>ASVHGTTYELLRRQGIDTVFGNPGSNELPFLKDFPEDFRYILALQEACVVGIADGYAQASRKPAFINLHSAAGTGNA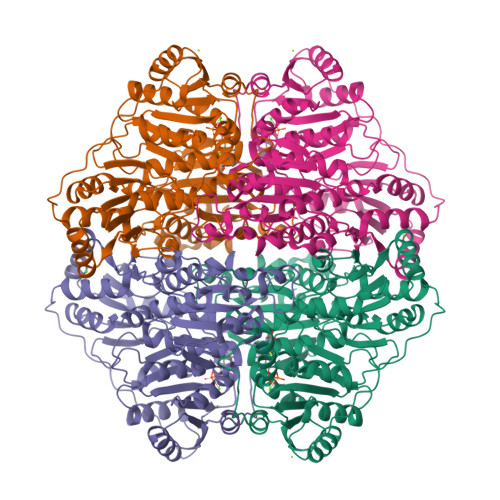MGALSNAWNSHSPLIVTAGQQTRAMIGVEALLTNVDAANLPRPLVKWSYEPASAAEVPHAMSRAIHMASMAPQGPVYLSVPYDDWDKDADPQSHHLFDRHVSSSVRLNDQDLDILVKALNSASNPAIVLGPDVDAANANADCVMLAERLKAPVWVAPSAPRCPFPTRHPCFRGLMPAGIAAISQLLEGHDVVLVIGAPVFRYHQYDPGQYLKPGTRLISVTCDPLEAARAPMGDAIVADIGAMASALANLVEESSRQLPTAAPEPAKVDQDAGRLHPETVFDTLNDMAPENAIYLNESTSTTAQMWQRLNMRNPGSYYFCAAGGLGFALPAAIGVQLAEPERQVIAVIGDGSANYSISALWTAAQYNIPTIFVIMNNGTYGALRWFAGVLEAENVPGLDVPGIDFRALAKGYGVQALKADNLEQLKGSLQEALSAKGPVLIEVSTVS[4x]>[2x]HHHHHHMNTINIAKNDFSDIELAAIPFNTLADHYGERLAREQLALEHESYEMGEARFRKMFERQLKAGEVADNAAAKPLITTLLPKMIARINDWFEEVKAKRGKRPTAFQFLQEIKPEAVAYITIKTTLACLTSADNTTVQAVASAIGRAIEDEARFGRIRDLEAKHFKKNVEEQLNKRVGHVYKKAFMQVVEADMLSKGLLGGEAWSSWHKEDSIHVGVRCIEMLIESTGMVSLHRQNAGVVGQDSETIELAPEYAEAIATRAGALAGISLMFQPCVVPPKPWTGITGGGYWANGRRPLALVRTHSKKALMRYEDVYMPEVYKA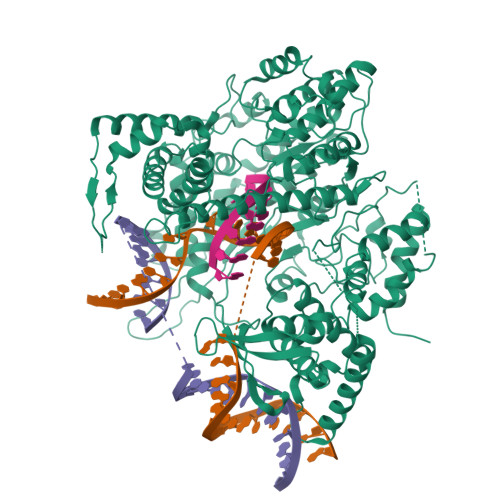INIAQNTAWKINKKVLAVANVITKWKHCPVEDIPAIEREELPMKPEDIDMNPEALTAWKRAAAAVYRKDKARKSRRISLEFMLEQANKFANHKAIWFPYNMDWRGRVYAVSMFNPQGNDMTKGLLTLAKGKPIGKEGYYWLKIHGANCAGVDKVPFPERIKFIEENHENIMACAKSPLENTWWAEQDSPFCFLAFCFEYAGVQHHGLSYNCSLPLAFDGSCSGIQHFSAMLRDEVGGRAVNLLPSETVQDIYGIVAKKVNEILQADAINGTDNEVVTVTDENTGEISEKVKLGTKALAGQWLAYGVTRSVTKRSVMTLAYGSKEFGFRQQVLEDTIQPAIDSGKGLMFTQPNQAAGYMAKLIWESVSVTVVAAVEAMNWLKSAAKLLAAEVKDKKTGEILRKRCAVHWVTPDGFPVWQEYKKPIQTRLNLMFLGQFRLQPTINTNKDSEIDAHKQESGIAPNFVHSQDGSHLRKTVVWAHEKYGIESFALIHDSFGTIPADAANLFKAVRETMVDTYESCDVLADFYDQFADQLHESQLDKMPALPAKGNLNLRDILESDFAFA5-[(phenylsulfonyl)amino]-1,3,4-thiadiazole-2-sulfonamide 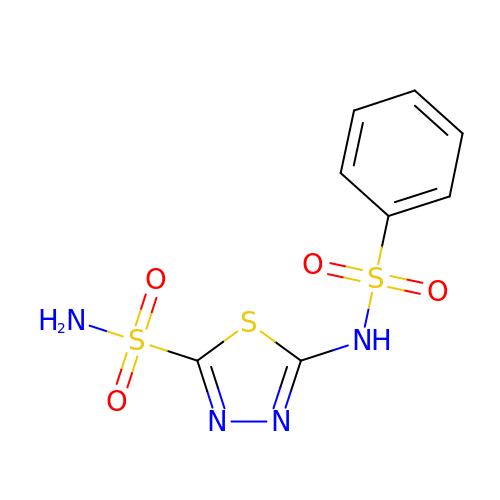| C8 H8 N4 O4 S3 | PWDGTQXZLNDOKS-UHFFFAOYSA-N>TTVYLAGDSTMAKNGGGSGTNGWGEYLASYLSATVVNDAVAGRSARSYTREGRFENIADVVTAGDYVIVEFGHNDGGSLSTDNGRTDCSGTGAEVCYSVYDGVNETILTFPAYLENAAKLFTAKGAKVILSSQTPNNPWETGTFVNSPTRFVEYAELAAEVAGVEYVDHWSYVDSIYETLGNATVNSYFP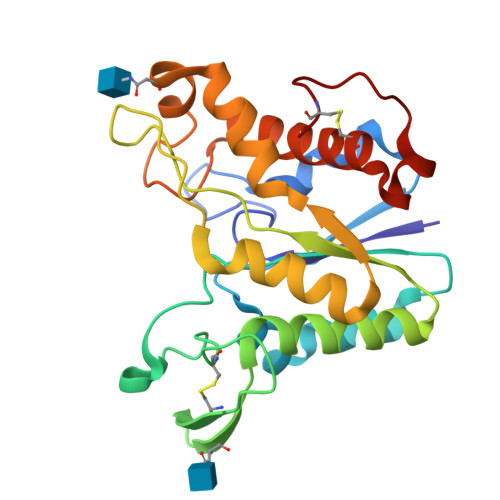IDHTHTSPAGAEVVAEAFLKAVVCTGTSLKSVLTTTSFEGTCL[2x]> GSKWKVFIDQINRSLENYEPCSSQNCSCYHGVIEEDLTPFRGGISRKMMAEVVRRKLGTHYQITKNRLYRENDCMFPSRCSGVEHFILEVIGRLPDMEMVINVRDYPQVPKWMEPAIPVFSFSKTSEYHDIMYPAWTFWEGGPAVWPIYPTGLGRWDLFREDLVRSAAQWPWKKKNSTAYFRGSRTSPERDPLILLSRKNPKLVDAEYTKNQAWKSMKDTLGKPAAKDVHLVDHCKYKYLFNFRGVAASFRFKHLFLCGSLVFHVGDEWLEFFYPQLKPWVHYIPVKTDLSNVQELLQFVKANDDVAQEIAERGSQFIRNHLQMDDITCYWENLLSEYSKFLSYNVTRRKGYDQIIP;> GSDGDQCASSPCQNGGSCKDQLQSYICFCLP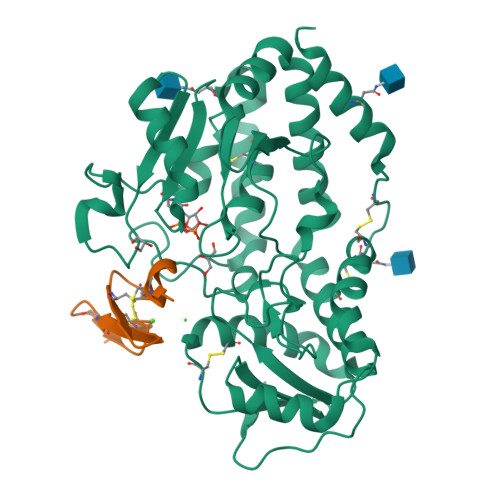AFEGRNCETHK>MIRTGTQYLESLNDGRNVWVGNEKIDNVATHPKTRDYAQRHADFYDLHHRPDLQDVMTYIDEGGQRRAMQWFGHRDKEQLRRKRKYHETVMREMAGASFPRTPDVNNYVLTTYIDDPAPWETQSIGDDGHIKAGKIVDFIRYAREHDLNCAPQFVDPQMDRSNPDAQERSPGLRVVEKNEKGIVVNGVKAIGTGVAFADWIHIGVFFRPGIPGDQVIFAATPVNTPGVTIVCRESLVKDDKVEHPLAAQGDELDGMTVFENVFIPWSHVFHIGNPNHAKLYPQRVFDWLHYHALIRQMVRAELVAGLAVLITEHIGTNKIPAVQTRVAKLIGFHQAMLAHLIASEELGFHTPGGHYKPNILIYDFGRALYLENFSQMIYELVDLSG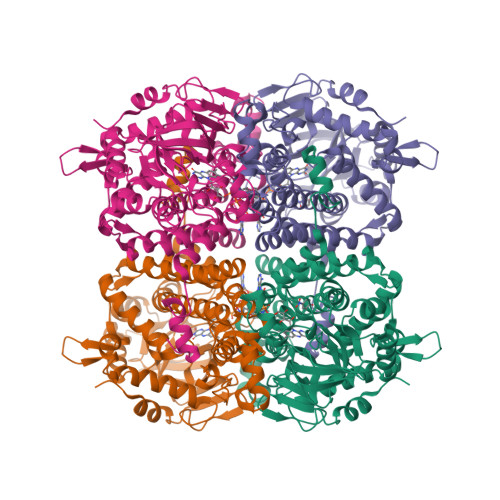RSALIFASEDQWNDDKLNGWFERMNNGPVGRPHDRVKIGRVIRDLFLTDWGSRLVVFENFNGTPLQGIRMLTMQRAEFSGSGPYGKLARQVCGIDSAVTDDTEYRKTADYAKALDAARHQEEVALAGAMAI[4x]>[2x]GSSHHHHHHMISRYTRPEMGAIWTEENKF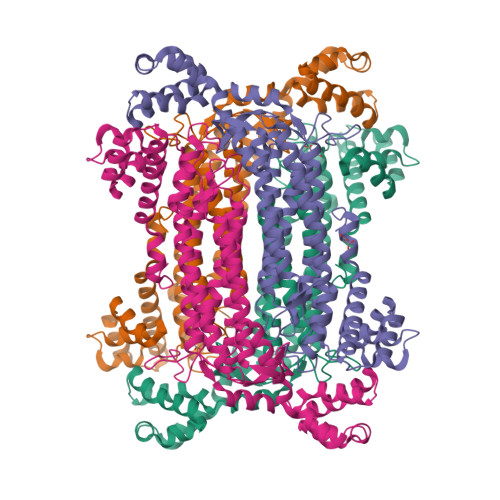KAWLEVEILACEAWAELGDIPKEDVKKIREHASFDIDRIYEIEKETRHDVVAFTRAVSETPALGEERKWVHYGLTSTDVVDTALSYILKQANEIILKDLENFVSILANKAKEHKYTIMMGRTHGVHAEPTTFGLKLGLWYEEMKRNVERFKQAANTVRVGKLSGAVGTYANIDPFVEKYVCENLGLEAAPISTQTLQRDRHAHYMSTLALIATSIEKMAVEIRGLQKSETREVEEAFAKGQKGSSAMPHKRNPIGSENMTGLARVIRGYMMTAYENVPLWHERDISHSSAERVILPDATIALNYMLNRFGNIVKNLTVYPENMKRNMTRTYGLIYSQRVMLTLIDKGMVREEAYDIVQPKAMEAWETQVQFKELVEADERITSKLTQEEINECFNYEHHMQHVDTIFERLGLNEA> AMAISNWVNVISDLKKIEDLIQSMHIDATLYTESDVHPSCKVTAMKCFLLELQVISLESGDASIHDTVENLIILANNSLSS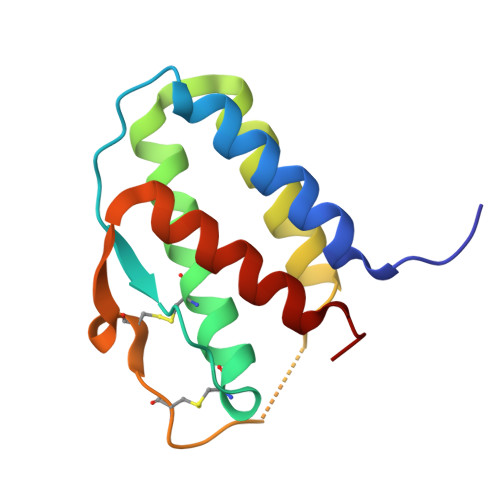NGNVTESGCKECEELEEKNIKEFLQSFVHIVQMFINTS>[14x]MSFPYFISPEQAMRERSELARKGIARAKSVVALAYAGGVLFVAE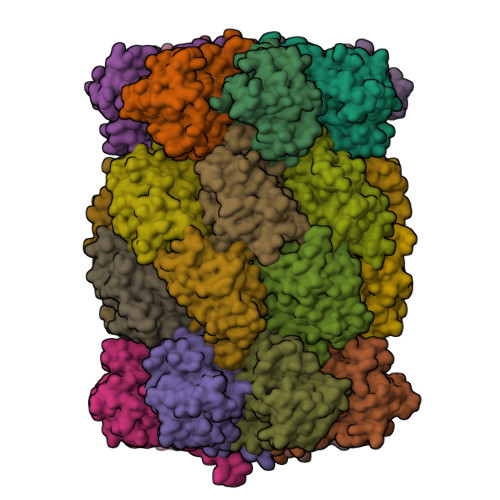NPSRSLQKISELYDRVGFAAAGKFNEFDNLRRGGIQFADTRGYAYDRRDVTGRQLANVYAQTLGTIFTEQAKPYEVELCVAEVAHYGETKRPELYRITYDGSIADEPHFVVMGGTTEPIANALKESYAENASLTDALRIAVAALRAGSADTSGGDQPTLGVASLEVAVLDANRPRRAFRRITGSALQALLVDQESPQSDGESSG;>[14x]MTWPLPDRLSINSLSGTPAVDLSSFTDFLRRQAPELLPASISGGAPLAGGDAQLPHGATIVALKYPGGVVMAGDRRSTQGNMISGRDVRKVYITDDYTATGIAGTAAVAVEFARLYAVELEHYEKLEGVPLTFAGKINRLAIMVRGNLAAAMQGLLALPLLAGYDIHASDPQSAGRIVSFDAAGGWNIEEEGYQAVGSGSLFAKSSMKKLYSQVTDGDSGLRVAVEALYDAADDDSATGGPDLVRGIFPTAVIIDADGAVDVPESRIAELARAIIESRSGADTFGSDGGEK> HHMQLEIQVALNFIISYLYNKLPRRRVNIFGEELERLLKKKYEGHWYPEKPYKGSGFRCIHIGEKVDPVIEQASKESGLDIDDVRGNLPQDLSVWIDPFEVSYQIGEKGPVKVLYVDDNNENGCELDKEIKNSFNPEAQVFMPISDPASSVSSSPSPPFGHSAAVSPTFMPRSTQPLTFTTATFAATKFGSTKMKNSGRSNKVARTSPINLGLNVNDLLKQKAISSSMHSLY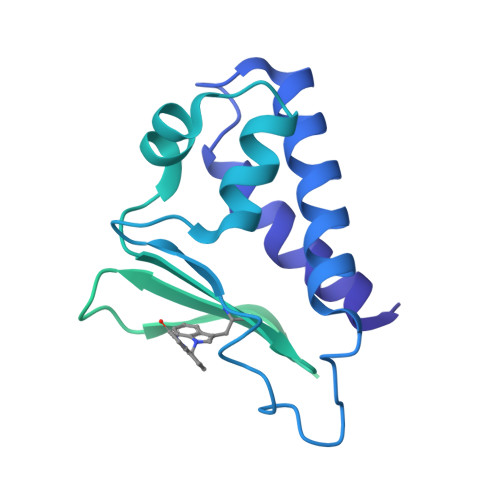GLGLGSQQQPQQQQQPAQPPPPPPPPQQQQQQKTSALSPNAKEFIFPNMQGQGSSTNGMFPGDSPLNLSPLQYSNAFDVFAAYGGLNEKSFVDGLNFSLNNMQYSNQQFQPVMAN> MARARGRGRRDLKSEINIVPLLDVLLVLLLIFMATAPIITQSVEVDLPDATESQAVSSNDNPPVIVEVSGIGQYTVVVEKDRLERLPPEQVVAEVSSRFKANPKTVFLIGGAKDVPYDEIIKALNLLHSAGVK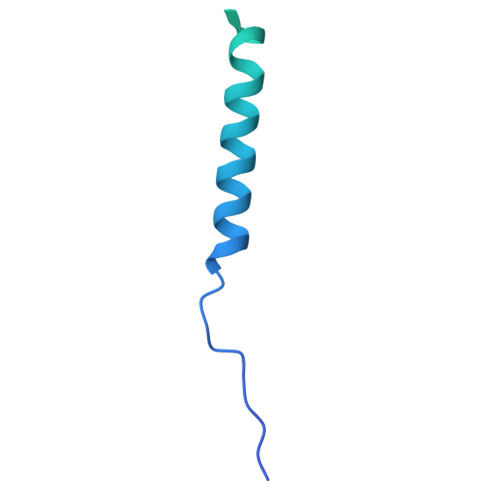SVGLMTQPI> MATKELKIGGVPVFPIFGGTAPVRQEGIMTQGDLVTVTSDGIDLNALWNSFAESIAIYNEAMDNLIQLLTYPVTVPVEPVVQIGETTFEEATELGVPRGAGLPIEVFQMGYDLRHYDKRN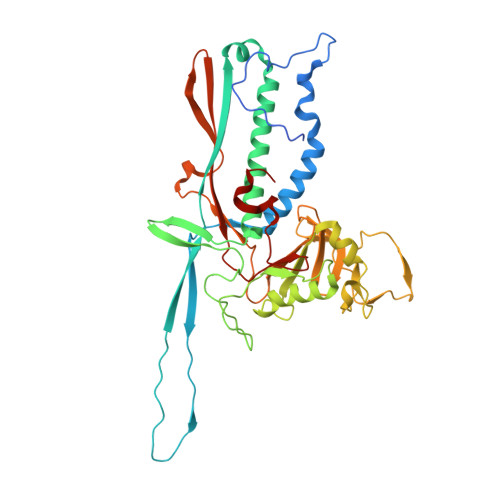AYSWMFLADADGRQVEAIHDAVLWADKRLVFRKVMEALFDNRTRRANIRNQAYNVYPLYNGDGVPPPRFKNNVFDETHSHYVISHNSVVDSSDLEDLMELLAEHGYSPQAGTQFLLLANKAETDAIRQFRRGVVNNNGATAGYDFIPSPTQPAMMLPNAEGLLGNQPAPTFGGLAVIGSYGFWNIVEEDYIPPGYLVGVGYGGAFNLGNPVGLRQHANPAMQGLRIIAGNYQRYPLVDGFYARSFGTGVRQRGGAAIMQIKASGAYECPPIYKKGGGFLV>[2x]ELTPDQQTLLHFIMDSYNKQRMPQEITNKILKEEFSAEENFLILTEMATNHVQVLVEF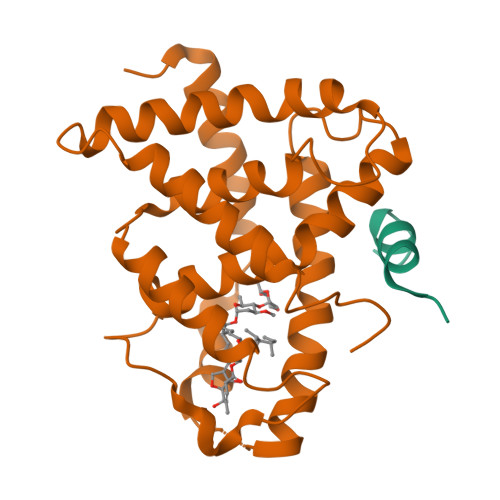TKKLPGFQTLDHEDQIALLKGSAVEAMFLRSAEIFNKKLPSGHSDLLEERIRNSGISDEYITPMFSFYKSIGELKMTQEEYALLTAIVILSPDRQYIKDREAVEKLQEPLLDVLQKLCKIHQPENPQHFACLLGRLTELRTFNHHHAEMLMSW;>[2x]SNLGLEDIIRKALMGSF>MLVKGNEILLKAHKEGYGVGAFNFVNFEMLNAIFEAGNEENSPLFIQASEGAIKYMGIDMAVGMVKIMCERYPHIPVALHLDHGTTFESCEKAVKAGFTSVMIDASHHAFEENLELTSKVVKMAHNAGVSVEAELGRLMGIEDNISVDEKDAVLVNPKEAEQFVKESQVDYLAPAIGTSHGAFKFKGEPKLDFERLQEVKRLTNIPLVLHGASAIPDNVRKSYLDAGGDLKGSKGVPFEFLQESVKG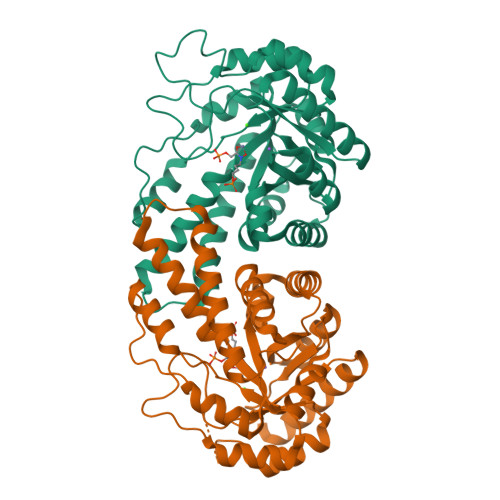GINKVNTDTDLRIAFIAEVRKVANEDKSQFDLRKFFSPAQLALKNVVKERMKLLGSANKI[2x]>PMTLGYWNIRGLAHSIRLLLEYTDSSYEEKKYTMGDAPDYDRSQWLNEKFKLGLDFPNLPYLIDGTHKITQSNAILRYIARKHNLCGESEKEQIREDILENQFMDSRMQLAKLCYDPDFEKLKPEYLQALPEMLKLYSQFLGKQPWFLGDKITFVDFIAYDVLERNQVFEPSCLDAFPNLKDFISRFEGLEKISAYMKSSRFLPR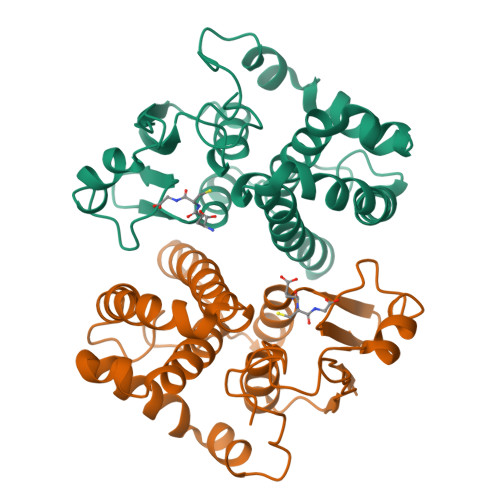PVFTKMAVFGNK[2x]> UUC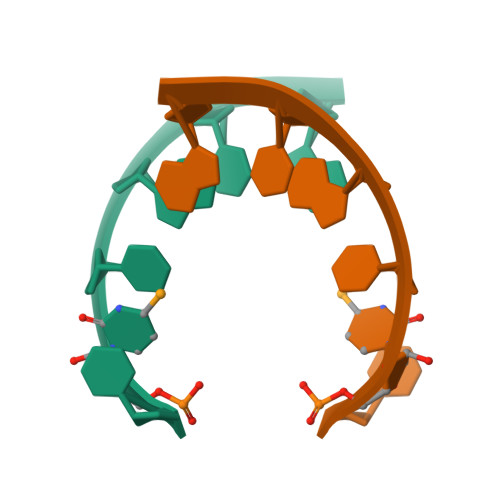GCG[[(2R)-1-(6-aminopurin-9-yl)propan-2-yl]oxymethyl-sulfanyl-phosphoryl] 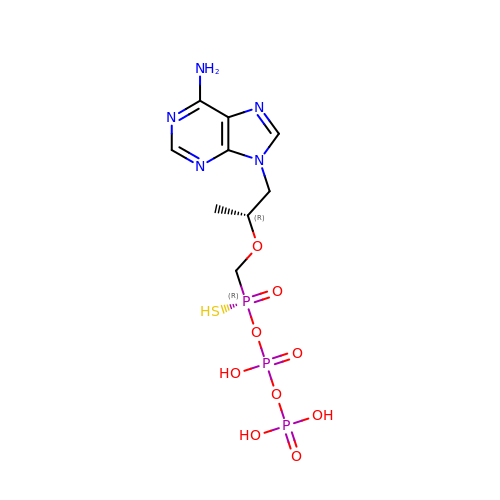phosphono hydrogen phosphate | C9 H16 N5 O9 P3 S | BMDSOWJDBWVWQG-FMWWOLKHSA-N>VLDGPYQPVAFKPPNDYWILVNSNSNGVVLEGTNNTDVWVAIISIEPNVNSESRQYSLFGVNKQITVVNTSNKWKFMEMFRNNSNAEFQHKRTLTSSTKLVGILKHGGRLWTYHGETPNATTDYSTTSNLNEISVTTYAEFYIIPRSQESKCTEYINTGL[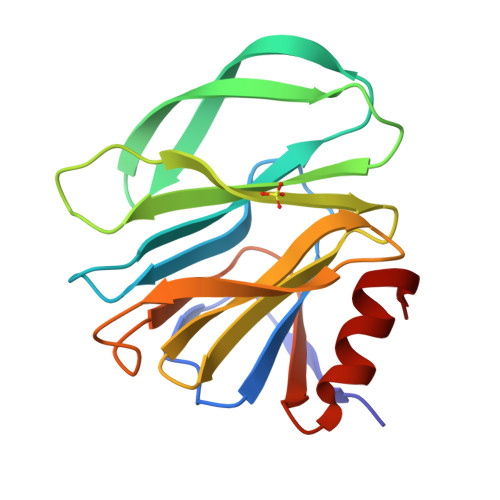8x]>[2x]HMGSAPGQKECDNALRQLETVRELLENPVQPINDMS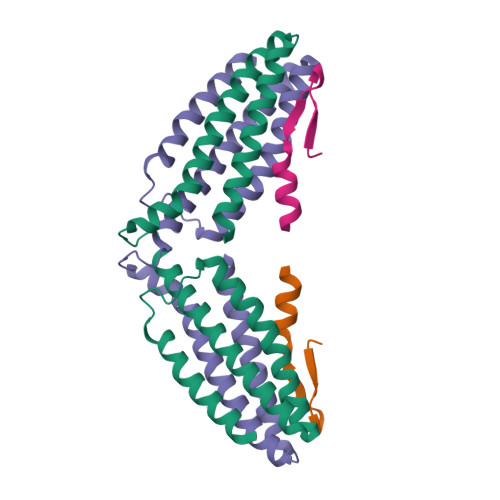YFGCLDSVMENSKVLGEAMTGISQNAKNGNLPEFGDAIATASKALCGFTEAAAQAAYLVGVSDPNSQAQISPEGRAAMEPIVISAKTMLESAGGLIQTARALAVNPRDPPRWSVLAGHSRTVSDSIKKLITSMRD;>[2x]PYFVETPYGYQLDLDFLKYVDDIQKG>GPLGSMAGGGAGDPGLGAAAAPAPETREHLFKVLVIGELGVGKTSIIKRYVHQLFSQHYRATIGVDFALKVLNWDSRTLVRLQLWDIAGLERFGNMTRVYYKEAVGAFVVFDISRSSTFEAVLKWKSDLDSKVHLPNGSPIPAVLLANKCDQNKDSSQSPSQVDQFCKEHGFAGWFETSAKDNINIEEAARFLVEKILVNHQSFPNEENDVDKIKLDQETLRAENKSQCC[3x];>[3x]GPLGSMDPSVVTPFSRDDRGHTPLHVAAVCGQASLIDLLVSKGAMVNATDYHGATPLHLACQKGYQSVTLLLLHYKASAEVQDNNGNTPLHLACTYGHEDCVKALVYYDVESCRLDIGNEKGDTPLHIAARWGYQGVIETLLQNGASTEIQNRLKETPLKCALNSKILSVMEAYHLSFERRQKSSEAPVQSPQRSVDHHHHHH

VARP is a Rab32/38 effector that also binds to the endosomal/lysosomal R-SNARE VAMP7. VARP binding regulates VAMP7 participation in SNARE complex formation and can therefore influence VAMP7-mediated membrane fusion events. Rab32 is an endosomal Rab GTPase, thought to have been present in the last eukaryotic common ancestor, with Rab38 arising in vertebrates as an evolutionary gene duplication of Rab32 (Klöpper et al., 2012). VARP has been shown to interact with Rab32/38 via its first ankyrin repeat-containing domain (Tamura et al., 2009, 2011; Wang et al., 2008).

We were able to crystallize a 1:1 complex of the smaller VARP fragment (residues 451–640) with the GTP hydrolysis-defective mutant of Rab32 (Q85L) in the presence of the nonhydrolyzable analog of GTP, GppCp. Its structure was solved at 2.8Å resolution by molecular replacement using VARP ANKRD2 and Rab7:GTP as search models. The final model comprises three molecules of the complex in the asymmetric unit, where VARP (residues 452–618), Rab32 (residues 22–198), and Rab32’s bound GppCp:Mg2+ are well defined in the electron density map. The three complexes in the asymmetric unit all have the same structure, with root-mean-square deviation (rmsd) values of 0.32 Å (for 306 Cα atoms of molecules A and B) and 0.33 Å (for 313 Cα atoms of molecules A and C). VARP ANKRD1 contains five tandem ankyrin repeats that form a slightly curved stack. The P loop (residues 32–39) stabilizes the Mg2+-coordinated triphosphate moiety of the nucleotide, while Switch-I (residues 48–61) folds over the nucleotide molecule and stabilizes the γ-phosphate of the GppCp. Switch-II (residues 84–97) also stabilizes the γ-phosphate but differs somewhat in conformation as compared to those in other GTP-bound Rab structures. The VARP ANKRD1:Rab32 heterodimer buries 1,530 Å2 of solvent accessible surface area (calculated with PISA; Krissinel and Henrick, 2007). The elongated interface consists of a central hydrophobic patch of residues from helices α2B (L513 and L514) and α3B (Y550 and Y551) of VARP and residues from Switch-I (V60), interswitch (F62, L69, and W80), and Switch-II (M91, V94, K97, and Y95) of Rab32. Flanking the hydrophobic core of the interface are two salt bridges formed through Switch-II of Rab32 (D480VARP-R93Rab32, H517VARP-K97Rab32) and a third one through the interswitch of the GTPase (K546VARP-D61Rab32).> GAMGIQCGGILVPMEDFARGAASPGPSRPGLVPVSIIGAEDEDFENELETNSEEQNSQFQSLEQVKRRPAHLMALLQHVALQFEPGPLLCCLHADMLGSLGPKEAKKAFLDFYHSFLEKTAVLRVPVPPNVAFELDRTRADLISEDVQRRFVQEV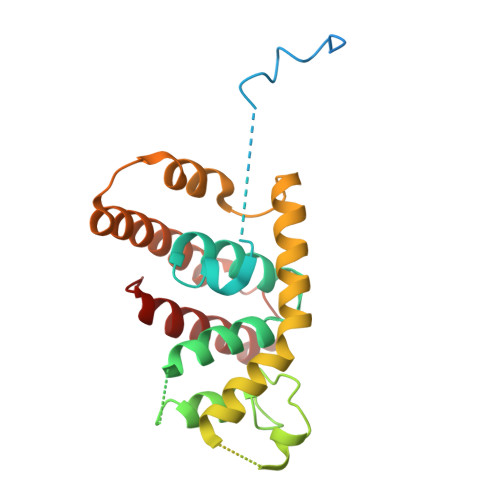VQSQQVAVGRQLEDFRSKRLMGMTPWEQELAQLEAWVGRDRASYEARERHVAERLLMHLEEMQHTISTDEEKSAAVVNAIGLYMRHLGVRT>MKLSLMVAISKNGVIGNGPDIPWSAKGEQLLFKAITYNQWLLVGRKTFESMGALPNRKYAVVTRSSFTSDNENVLIFPSIKDALTNLKKITDHVIVSGGGEIYKSLIDQVDTLHISTIDIEPEGDVYFPEIPSNFRPVFTQDFAS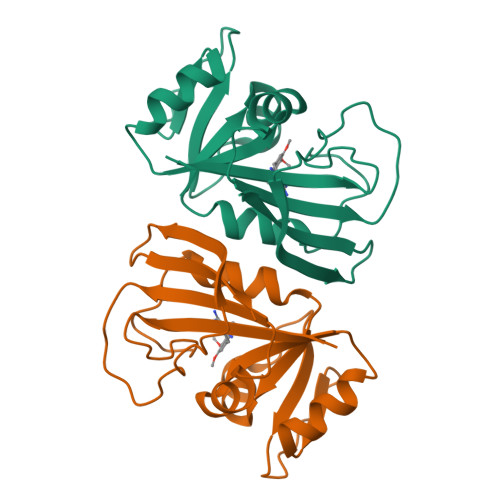NINYSYQIWQKGLEHH[6x]> AASGVATNTPTANDEEYITPVTIGGTTLNLNFDTGSADLWVFSTELPASQQSGHSVYNPSATGKELSGYTWSISYGDGSSASGNVFTDSVTVGGVTAHGQAVQAAQQISAQFQQDTNNDGLLGLAFSSINTVQPQSQTTFFDTVKSSLAQPLFAVALKHQQPGVYDFG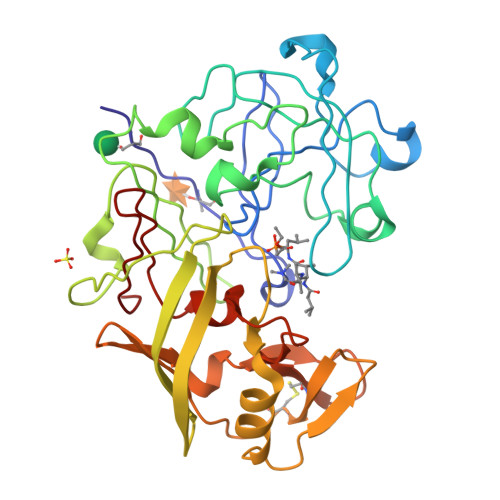FIDSSKYTGSLTYTGVDNSQGFWSFNVDSYTAGSQSGDGFSGIADTGTTLLLLDDSVVSQYYSQVSGAQQDSNAGGYVFDCSTNLPDFSVSISGYTATVPGSLINYGPSGDGSTCLGGIQSNSGIGFSIFGDIFLKSQYVVFDSDGPQLGFAPQA> VVGGTDADEGEWPWQVSLHALGQGHICGASLISPNWLVSAAHCYIDDRGFRYSDPTQWTAFLGLHDQSQRSAPGVQERRLKRIISHPFFNDFTFDYDIALLELEKPAEYSSMVRPICLPDASHVFPAGKAIWVTGWGHTQYGGTGALILQKGEIRVIQQTTCENLLPQQITPRMMCVGFLSGGVDSCQGDSGGPLSSVEADGRIFQAGVVSWGDGCAQRNKPGVYTRLPLFRDWIKENTGV;> GRCTKSIPPICFPD

Matriptase is a type II transmembrane serine protease that is found on the surfaces of epithelial cells and certain cancer cells. Matriptase has been implicated in the degradation of certain extracellular matrix components as well as the activation of various cellular proteins and proteases, including hepatocyte growth factor and urokinase. Matriptase activity is down-regulated by its physiological inhibitor, hepatocyte growth factor activator inhibitor-1 (HAI-1). Sunflower trypsin inhibitor-1 (SFTI-1), a cyclic peptide inhibitor originally isolated from sunflower seeds, exhibits potent inhibitory activity toward matriptase.

The crystal structure of β-matriptase-N164Q in complex with SFTI-1 was solved at 2.0 Å. In this structure, SFTI-1 forms a bicyclic structure where two antiparallel β-strands are constrained by a disulfide bond between Cys3 and Cys11. The cyclic peptidic inhibitor docks onto matriptase's P4-P2' specificity sites with good shape and charge complementarity. The SFTI-1 scissile bond (Lys5-Ser6) is in close proximity to the catalytic residue Ser195 where the Ser195 hydroxyl group hydrogen bonds with the main-chain amide of Ser6 and makes close contacts with the backbone carbonyl and amide of Lys5 (2.9Å and 3.0 Å respectively). The side chain oxygen atom of Ser195 is also in close contact with the carbonyl carbon of P1 residue (Lys5) (2.6 Å) at an angle of 88.6° (Lys5O-C-Ser195OG), suggesting the protease is in an active conformation capable of initiating bond scission. Furthermore, His57 is suitably oriented to interact with Ser195 to support catalysis (at 2.6 Å and with Ser195CB-OG-His57NE2 angle of 101.4°). These observations support that SFTI-1 functions as a substrate variant of matriptase in a similar manner to other BBIs. In the structure, the S2 subsite of matriptase is occupied by SFTI-1 Thr4 with Thr4 side chain flanked by His57 and Phe99. Comparing to the benzamidine-bound structure, we observed that the benzyl ring of Phe99 undergoes a rotation to widen the pocket to better accommodate the P2 residue. More importantly, the guanidinium group of Arg2 forms cation-π interactions with both phenylalanines as well as Trp215 in T-shaped geometries and provides further stabilization.>[2x]GNGILSSLYDEPETAKDFGFITIDHANHSGTVRVDATQYTKWNYINLHTLQIDSAKVTAEGADDPDTWDLAIHRYDVKTNGGEVLETDYQSLSALKNAGSMPQGIFVADEWTTNKIA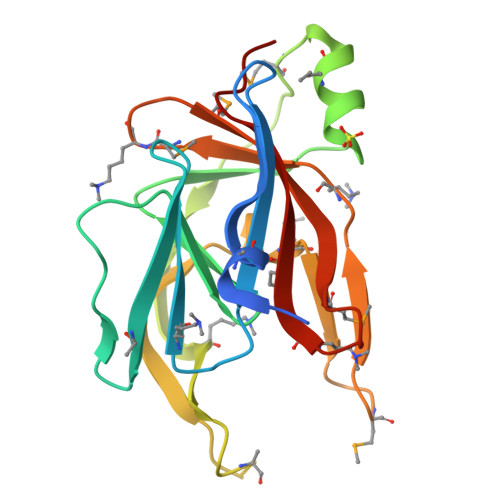VDVSHMMEDNGYLIYAPSDFNPELSKWLNVDTSEMPPIYTPSNKVYLLRMKDDTMAAIRLVSYMNAAGIKGYMTFDYIYPYEP> M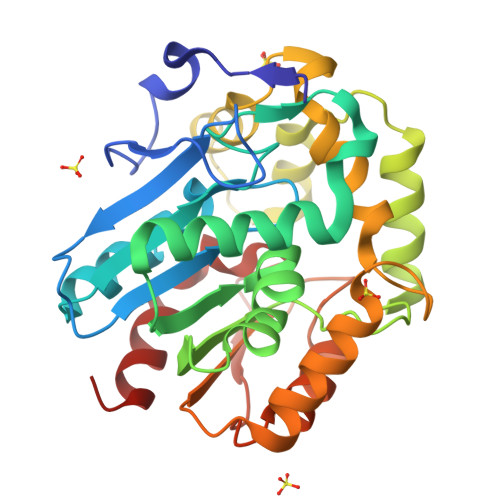EFVRTPDDRFADLPDFPYAPHYLEGLPGFEGLRMHYVDEGPRDAEHTFLCLHGEPSWSFLYRKMLPVFTAAGGRVVAPDLFGFGRSDKPTDDAVYTFGFHRRSLLAFLDALQLERVTLVCQDWGGILGLTLPVDRPQLVDRLIVMNTALAVGLSPGKGFESWRDFVANSPDLDVGKLMQRAIPGITDAEVAAYDAPFPGPEFKAGVRRFPAIVPITPDMEGAEIGRQAMSFWSTQWSGPTFMAVGAQDPVLGPEVMGMLRQAIRGCPEPMIVEAGGHFVQEHGEPIARAALAAFGQ> EHQLLRYLLD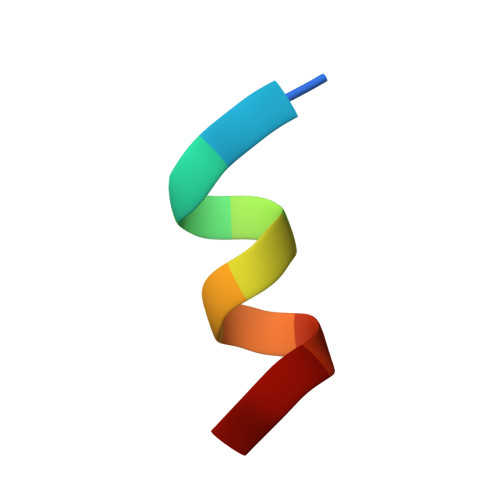K> GSSMGSLNQDATILRQAKLGLSDPAQSLSSWSDNNDVTPCKWLGVSCDATSNVVSVDLSSFMLVGPFPSILCHLPSLHSLSLYNNSINGSLSADDFDTCHNLISLDLSENLLVGSIPKSLPFNLPNLKFLEISGNNLSDTIPSSFGEFRKLESLNL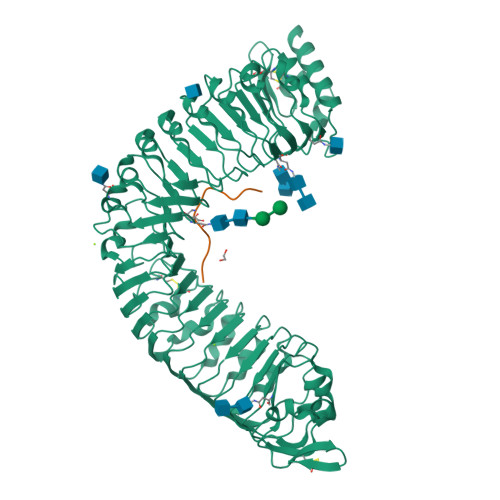AGNFLSGTIPASLGNVTTLKELKLAYNLFSPSQIPSQLGNLTELQVLWLAGCNLVGPIPPSLSRLTSLVNLDLTFNQLTGSIPSWITQLKTVEQIELFNNSFSGELPESMGNMTTLKRFDASMNKLTGKIPDNLNLLNLESLNLFENMLEGPLPESITRSKTLSELKLFNNRLTGVLPSQLGANSPLQYVDLSYNRFSGEIPANVCGEGKLEYLILIDNSFSGEISNNLGKCKSLTRVRLSNNKLSGQIPHGFWGLPRLSLLELSDNSFTGSIPKTIIGAKNLSNLRISKNRFSGSIPNEIGSLNGIIEISGAENDFSGEIPESLVKLKQLSRLDLSKNQLSGEIPRELRGWKNLNELNLANNHLSGEIPKEVGILPVLNYLDLSSNQFSGEIPLELQNLKLNVLNLSYNHLSGKIPPLYANKIYAHDFIGNPGLCVDLDGLCRKITRSKLEGSENLYFQ;> PIPPSAPSKRHN>MKELIRKLTEAFGPSGREEEVRSIILEELEGHIDGHRIDGLGNLIVWKGSGEKKVILDAAIDEIGVVVTNVDDKGFLTIEPVGGVSPYMLLGKRIRFENGTIGVVGMEGETTEERQENVRKLSFDKLFIDIGANSREEAQKMCPIGSFGVYDSGFVEVSGKYVSKAMDDRIGCAVIVEVFKRIKPAVTLYGVFSVQEEVGLVGASVAGYGVPADEAIAIDVTDSADTPKAIKRHAMRLSGGPALKVKDRASISSKRILENLIEIAEKFDIKYQME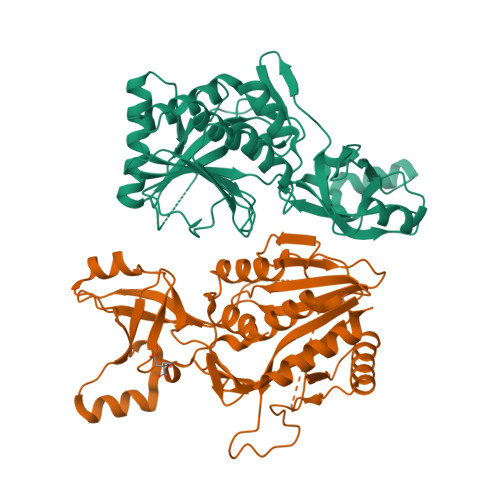VLTFGGTNAMGYQRTREGIPSATVSIPTRYVHSPSEMIAPDDVEATVDLLIRYLGA[2x]> NLQQFKNMIQCAGTRTWTAYINYG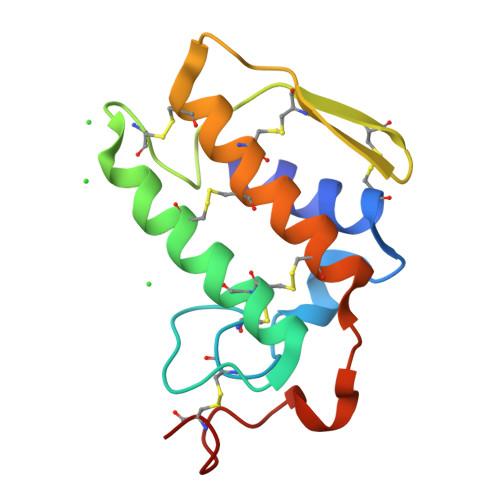CYCGKGGSGTPVDKLDRCCYTHDHCYNQADSIPGCNPNIKTYSYTCTQPNITCTRTADACAKFLCDCDRTAAICFASAPYNINNIMISASNSCQ s-citryldethia Coenzyme A | C28 H46 N7 O22 P3 | 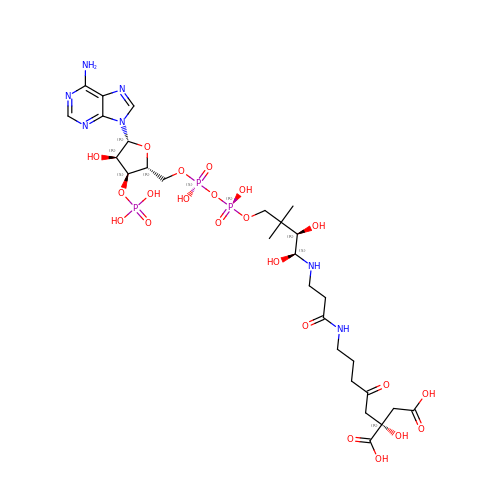JCKIRWYQPYQCEC-LWCHDFGBSA-N>MAPVLSKDVADIESILALNPRTQSHAALHSTLAKKLDKKHWKRNPDKNCFHCEKLENNFDDIKHTTLGERGALREAMRCLKCADAPCQKSCPTHLDIKSFITSISNKNYYGAAKMIFSDNPLGLTCGMVCPTSDLCVGGCNLYATEEGSINIGGLQQFASEVFKAMNIPQIRNPCLPSQEKMPEAYSAKIALLGAGPASISCASFLARLGYSDITIFEKQEYVGGLSTSEIPQFRLPYDVVNFEIELMKDLGVKIICGKSLSENEITLNTLKEEGYKAAFIGIGLPEPKTDDIFQGLTQDQGFYTSKDFLPLVAKSSKAGMCACHSPLPSIRGAVIVLGAGDTAFDCATSALRCGARRVFLVFRKGFVNIRAVPEEVELAKEEKCEFLPFLSPRKVIVKGGRIVAVQFVRTEQDETGKWNEDEDQIVHLKADVVISAFGSV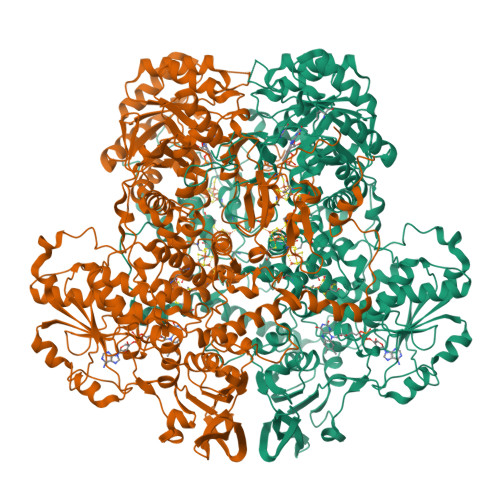LRDPKVKEALSPIKFNRWDLPEVDPETMQTSEPWVFAGGDIVGMANTTVESVNDGKQASWYIHKYIQAQYGASVSAKPELPLFYTPVDLVDISVEMAGLKFINPFGLASAAPTTSSSMIRRAFEAGWGFALTKTFSLDKDIVTNVSPRIVRGTTSGPMYGPGQSSFLNIELISEKTAAYWCQSVTELKADFPDNIVIASIMCSYNKNDWMELSRKAEASGADALELNLSAPHGMGERGMGLACGQDPELVRNICRWVRQAVQIPFFAKLTPNVTDIVSIARAAKEGGADGVTATNTVSGLMGLKADGTPWPAVGAGKRTTYGGVSGTAIRPIALRAVTTIARALPGFPILATGGIDSAESGLQFLHSGASVLQVCSAVQNQDFTVIQDYCTGLKALLYLKSIEELQGWDGQSPGTESHQKGKPVPRIAELMGKKLPNFGPYLEQRKKIIAEEKMRLKEQNAAFPPLERKPFIPKKPIPAIKDVIGKALQYLGTFGELSNIEQVVAVIDEEMCINCGKCYMTCNDSGYQAIQFDPETHLPTVTDTCTGCTLCLSVCPIIDCIRMVSRTTPYEPKRGLPLAVNPVC[4x]>[8x]MRVENNNVSGQNHDPEQIDLIDLLVQLWRGKMTIIISVIVAIALAIGYLAVAKEKWTSTAIITQPDVGQIAGYNNAMNVIYGQAAPKVSDLQETLIGRFSSAFSALAETLDNQEEREKLTIEPSVKNQQLPLTVSYVGQTAEGAQMKLAQYIQQVDDKVNQELEKDLKDNIALGRKNLQDSLRTQEVVAQEQKDLRIRQIQEALQYANQAQVTKPQI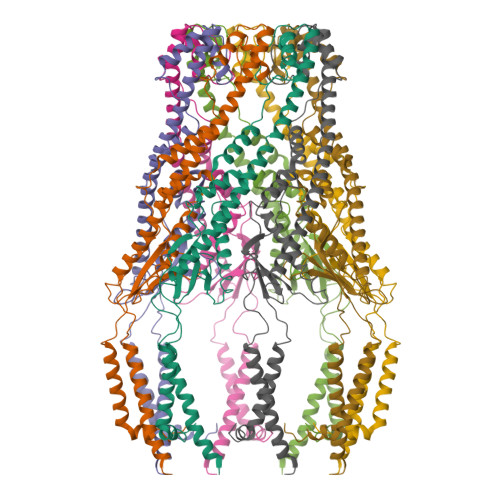QQTGEDITQDTLFLLGSEALESMIKHEATRPLVFSPNYYQTRQNLLDIESLKVDDLDIHAYRYVMKPMLPIRRDSPKKAITLILAVLLGGMVGAGIVLGRNALRNYNAKEFRVPGSHHHHHHHH>[4x]LDGDQMISHRELWAKIANSINDINEYLKVYEHAVSSYTQMYQDFSAVLSSLAGWISPGGNDGNSVKLQVNSLKKALEELKEKYKDKPLYPANNTVSQEQANKWLTELGGTIGKVSQKNGGYVVSINMTPIDNMLKSLDNLGGNGEVVLDNAKYQAWNAGFSAEDETMKNNLQTLVQKYSNANSIFDNLVKVLSSTISS

Like many Gram-negative pathogens, Shigella rely on their type three secretion system (T3SS) to inject effector proteins into eukaryotic host cells, driving both cellular invasion and evasion of host immune responses. Studies in Shigella have demonstrated that bile salts found in the small intestine (e.g., deoxycholate (DOC)) interact directly with the injectisome tip complex protein invasion plasmid antigen D (IpaD) to support interaction with the hydrophobic translocator protein IpaB and its stable recruitment to the maturing tip complex. In Shigella, IpaD resides at the extracellular tip of the injectisome where it functions as a “gatekeeper” that prevents unwanted protein secretion (leakage) through the injectisome prior to requisite activation events. Here, we uncover critical mechanistic details of the Shigella-specific DOC signaling process by describing the role of a π-helix secondary structure element within the T3SS tip protein invasion plasmid antigen D (IpaD).

Here, we mimicked the previously successful native proteolytic cleavage by engineering IpaDWT, IpaDΔQ148, and IpaDΔY149 to lack their N terminal 121 residues. These N-terminal truncation constructs expressed and purified well in E. coli and diffracting crystals of IpaDΔ1–121, WT and IpaDΔ1–121, ΔQ148 formed overnight by vapor diffusion. The IpaDΔ1–121, ΔQ148 structure clearly shows that the π-helix has been eliminated through conversion of the surrounding region to an α-helix. When the proximal (bottom) regions of the structures are aligned, a modest translation of the distal portion of the structure is observed in the mutant relative to that of the WT. Importantly, however, elimination of the π-helix does not impact the registry of the surrounding residues or significantly alter the positioning of the adjacent side chains, supporting the feasibility of this mutant as a means to independently dissect the role of the π-helix in IpaD. Fortunately, a 3.00 Å structure of IpaDΔQ148 verified the removal of the π-helix (conversion to α-helix) and minimal impact on the global structure of the mutant, consistent with the CD data for both constructs. Aligning the IpaDΔ1–121, WT and IpaDΔ1–121, ΔQ148 structures additionally shows that Y149 sterically prevents the F308 rotamer change in the WT π-helix structure. However, removing the π-helix moves the tyrosine side chain approximately 2.4 Å away from the helix interface and the phenylalanine is no longer prevented from adopting the necessary rotamer conformation that supports DOC binding in this region.> ANIVGGIEYSINNASLCSVGFSVTRGATKGFVTA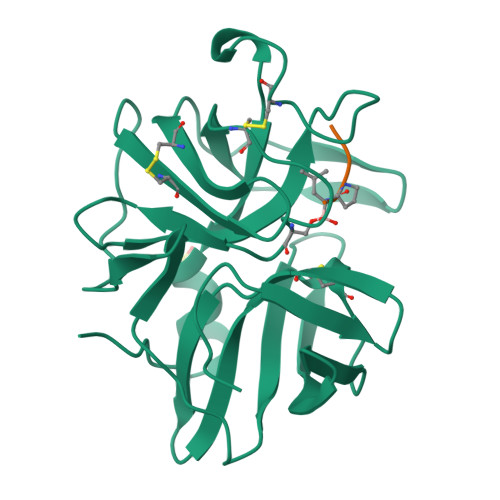GHCGTVNATARIGGAVVGTFAARVFPGNDRAWVSLTSAQTLLPRVANGSSFVTVRGSTEAAVGAAVCRSGRTTGYQCGTITAKNVTANYAEGAVRGLTQGNACAGRGDSGGSWITSAGQAQGVMSGGNVQSNGNNCGIPASQRSSLFERLQPILSQYGLSLVTG;> XAAPL> IHEGILFCIELSETMFKESSDLEYKSPLLEILESLDELMSQLVITRPGTAIGCYFYYCNREDAKEGIYELFPLRDINATFMKKLNDLLEDLSSGRISLYDYFMFQQTGSEKQVRLSVLFTFMLDTFLEEIPGQKQLSNKRVFLFTDIDKPQEAQDIDERARLRRLTIDLFDNKVNFATFFIGYADKPFDNEFYSDILQLGSHTNENTGLDSEFDGPSTKPIDAKYIKSRILRKKEVKRIMFQCPLILDEKTNFIVGV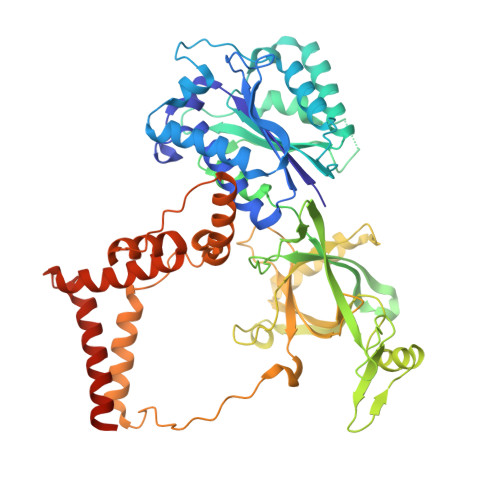KGYTMYTHEKAGVRYKLVYEHEDIRQEAYSKRKFLNPITGEDVTGKTVKVYPYGDLDINLSDSQDQIVMEAYTQKDAFLKIIGFRSSSKSIHYFNNIDKSSFIVPDEAKYEGSIRTLASLLKILRKKDKIAILWGKLKSNSHPSLYTLSPSSVKDYNEGFYLYRVPFLDEIRKFPSLLSYDDGSEHKLDYDNMKKVTQSIMGYFNLRDGYNPSDFKNPLLQKHYKVLHDYLLQIETTFDENETPNTKKDRMMREDDSLRKLYYIRNKILESEKSEDPIIQRLNKYVKIWNMFYKKFNDDNISIKEEKKPFDKKPKFNI> GDVGAGEQIFNANCAACHAG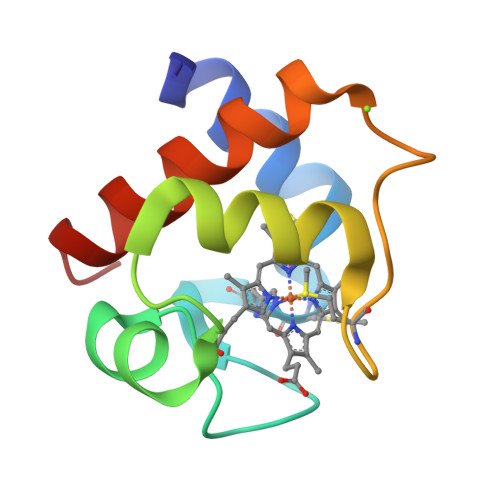GQNVIMPEKTLEKEALDQYLAGGRTEKSIISQVTGGKNAMPAFGGRLSDEEIANVAAYVLASAEAGWE> AHPETLVKVKDAKDQLGKRVGYIELDLASGKILVSFRPEERFPMMSTFKVLLCGAVLSRVDAGQEQLGRRIHYSQNDLVEYSPVTEKHLTDGMTVGELCSAAITMSDNTAANLLLTTIGGPKELTAFLHNMGDHVTRLDRWEPELNEAIPNDERDTTTPVAMATTLRKLLTGELLTAASRQQLIDWMEADKVAGPLLRSAL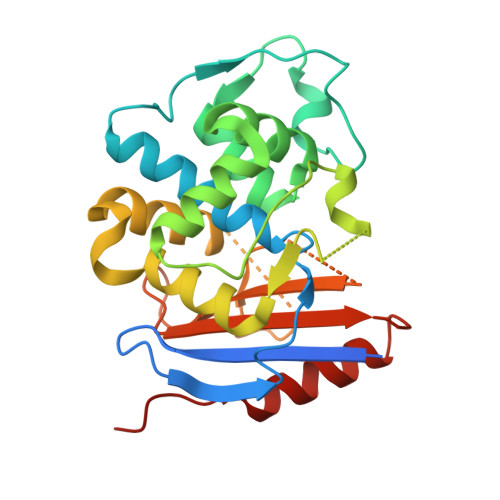PAGWFIADKSGAGERGSRGIIAALGPDGKPSRIVVIYMTGSQATMDERNRQIAEIGASLIKHWA> MLIQAVGVNLPPSYVCLEGPLGGERPRAQGDEMLMQRLLPAVREALDEAAVKPEEIDLIVGLALSPDHLIENRDIMAPKIGHPL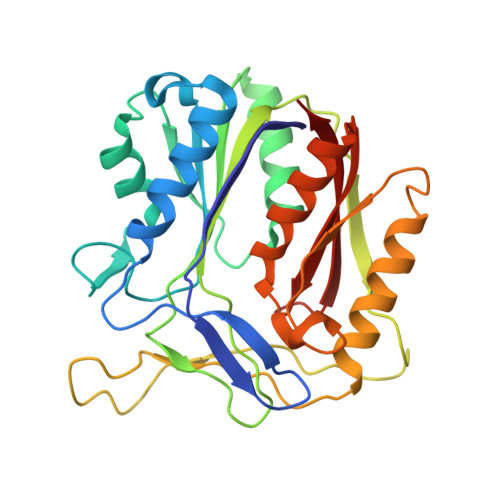QKVLGANRAHVFDLTDSSLARALYVVDTLASDQGYRNVLVVRGESSQGLEVDSESGFALADGALALLCRPTGKAAFRRGALGGDPAQEWLPLSIPLNTDIRQVGDVKGHLNLPAQPGLPEAVRAGFTRLAGDFPQLNWVREEWFGQGRPDGRCLGPFELASQLRAAQRDRLDELLLISFDPFGMVVEGVTLELAGEAHA rabelomycin | C19 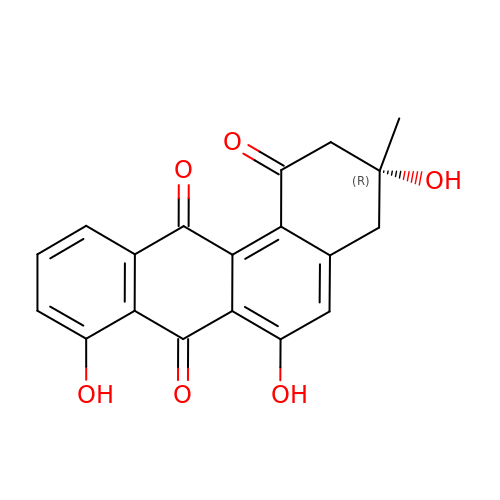H14 O6 | JJOLHRYZQSDLSA-LJQANCHMSA-N>[2x]MDLT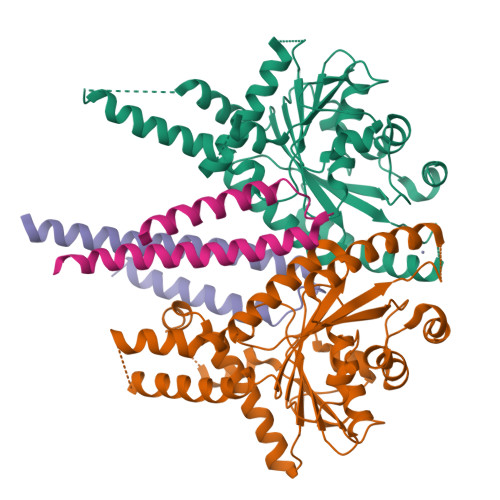VEPNLHSLITSTTHKWIFVGGKGGVGKTTSSCSIAIQMALSQPNKQFLLISTDPAHNLSDAFGEKFGKDARKVTGMNNLSCMEIDPSAALKDMNDMAVSRANNNGSDGQGDDLGSLLQGGALADLTGSIPGIDEALSFMEVMKHIKRQEQGEGETFDTVIFDTAPTGHTLRFLQLPNTLSKLLEKFGEITNKLGPMLNSFMGAGNVDISGKLNELKANVETIRQQFTDPDLTTFVCVCISEFLSLYETERLIQELISYDMDVNSIIVNQLLFAENDQEHNCKRCQARWKMQKKYLDQIDELYEDFHVVKMPLCAGEIRGLNNLTKFSQFLNKEYNPITDGKVIYELEDKE;>TNKYHEKWISKFAPGNELSKKYLAKVKERHELKEFNNSISAQDNYAKWTKNNRKLDSLDKEINNLKDEIQSENKAFQAHLHKLR[2x]>MVIASVEDGGDGDTSKDDWLWYKQPASQTDATATAGGNYGNPDNNRWQQTTLPFGNGKIGGTVWGEVSRERVTFNEETLWTGGPGSSTSYNGGNNETKGQNGATLRALNKQLANGAETVNPGNLTGGENAAEQGNYLNWGDIYLDYGFNDTTVTEYRRDLNLSKGKADVTFKHDGVTYTREYFASNPDNVMVARLTASKAGKLNFNVSMPTNTNYSKTGETTTVKGDTLTVKGALGNNGLLYNSQIKVVLDNGEGTLSEGSDGASLKVSDAKAVTLYIAAATDYKQKYPSYRTGETAAEVNTRVAKVVQDAANKGYTAVKKAHIDDHSAIYDRVKIDLGQSGHSSDGAVATDALLKAYQRGSATTAQKRELETLVYKYGRYLTIGSSRENSQLPSNLQGIWSVTAGDNAHGNTPWGSDFHMNVNLQMNYWPTYSANMGELAEPLIEYVEGLVKPGRVTAKVYAGAETTNPETTPIGEGEGYMAHTENTAYGWTAPGQSFSWGWSPAAVPWILQNVYEAYEYSGDPALLDRVYALLKEESHFYVNYMLHKAGSSSGDRLTTGVAYSPAQGPLGTDGNTYESSLVWQMLNDAIEAAKAKGDPDGLVGNTTDCSADNWAKNDSGNFTDANANRSWSCAKSLLKPIEVGDSGQIKEWYFEGALGKKKDGSTISGYQADNQHRHMSHLLGLFPGDLITIDNSEYMDAAKTSLRYRCFKGNVLQSNTGWAIGQRINSWARTGDGNTTYQLVELQLKNAMYANLFDYHAPFQIDGNFGNTSGVDEMLLQSNSTFTDTAGKKYVNYTNILPALPDAWAGGSVSGLVARGNFTVGTTWKNGKATEVRLTSNKGKQAAVKITA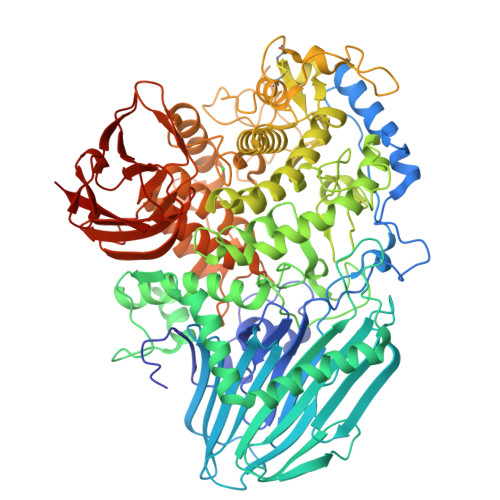GGAQNYEVKNGDTAVNAKVVTNADGASLLVFDTTAGTTYTITKKAS[2x]>[2x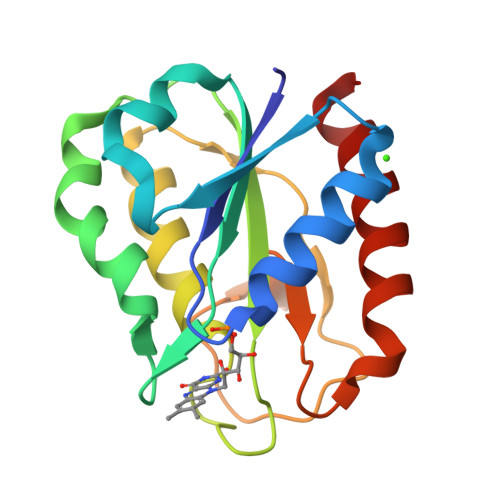]SKKIGLFYGTQTGKTKSVAEIIRDEFGNDVVTLHDVSQAEVTDLNDYQYLIIGCPTWNIGKLQSDWEGLYSELDDVDFNGKLVAYFGTGDQIGYADNFQDAIGILEEKISQRGGKTVGYWSTDGYKFNDSKALRNGKFVGLALDEDNQSKLTDDRIKSWVAQLKSEFGL> MSPYSSDTTPCCAAAIARPLPRAHIKEYFYTSGKCSNPAVVFVTRKNRQVCANPEKKWVREYINSLEMS

CC-type chemokine ligand 5 (CCL5) also known as RANTES (regulated on activation, normal T cell expressed and secreted) is expressed and produced by many types of cells including platelets, macrophages, eosinophils, fibroblasts, and epithelial cells. The molecule participates in a wide range of inflammatory disorders and pathologies. There are at least three phases for CCL5 oligomerization and aggregation that depend on pH, concentration, and temperature. By multiple sequence alignments of CCL5s from different animals, CCL5s conversely compose the sequence of F12-A13-Y14 (12FAY14).

The CCL5 variant, CCL5-12AAA14 with two Ala substitutions at residues F12 and Y14, resulted in the formation of a less aggregated mutant. Therefore, we were able to crystalize the sulfate-stabilized CCL5-12AAA14. The crystals belong to the trigonal space group P3121 with unit-cell parameters a = b = 48.3 Å and c = 60.4 Å and a solvent content of 54%. The structure of CCL5-12AAA14 monomer was refined to 2.55 Å. The structure of the CCL5-12AAA14 monomer matched the generalized view of a typical chemokine tertiary structure, consisting of an extended N-terminal portion (N–P20), a short 310 helix (R21–H23), a triple-stranded antiparallel β-sheet (β1: I24–F28, β2: V39–T43, and β3: N46–A51) and a C-terminal α-helix (α1: K56–E66). Notably, although one CCL5-12AAA14 molecule existed in one asymmetric unit, it packed as a dimer with two-fold symmetry. In the interface of the CCL5-12AAA14 dimer, backbone hydrogen bonds were formed between C10 (chain A) and C10′ (chain B), T7 and C50′, and T8 and Q48′. There is a one-residue shifting in the N-terminal backbone pairing region, which changes the relative orientation of the two monomers. The overall length and size of the CCL5-12AAA14 dimer becomes shorter and more compact, while the distance becomes closer between the two α1 elements. The native CCL5 cannot adopt the CCL5-12AAA14 dimer configuration because the sidechains of F12 and F12′ are too close to pack together in the structure.> MKTINSVDTKEFLNHQVANLNVFTVKIHQIHWYMRGHNFFTLHEKMDDLYSEFGEQMDEVAER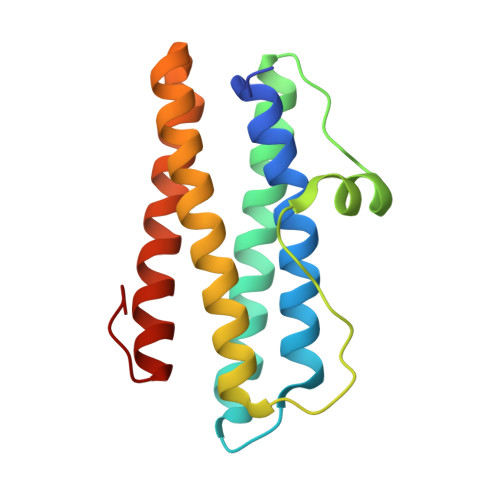LLAIGGSPFSTLKEFLENASVEEAPYTKPKTMDQLMEDLVGTLELLRDEYKQGIELTDKEGDDVTNDMLIAFKASIDKHIWMFKAFLGKAPLE>MQMAKVCGTVVGTQKLPSMTGVKLLLLQFIDANGELLPKYEVAADPVGAGLGEWVLVNRGSAARQTEYHQNRPLDAMVVAIIDTVTVNNRRLYGEGSWSHPQFEK[60x];>MAVAVGMIETLGFPAVVEAADAMVKAARVTLVGYEKIGTGRVTVIVRGDVSEVQASVSAGTESVKRVNGGQVLSTHIIARPHEN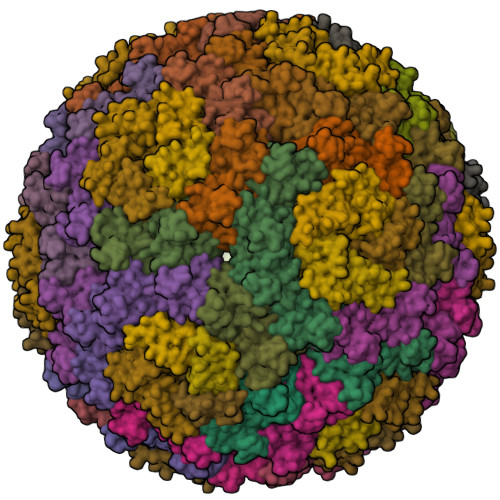LEYVLPIRYTEEVEQFREGVGTPRNITRQ[120x]>[2x]PNVAIIVAALKPALGIGYKGKMPWRLRKEIRYFKDVTTRTTKPNTRNAVIMGRKTWESIPQKFRPLP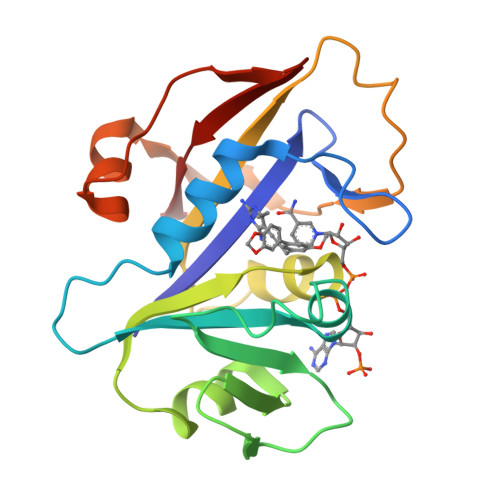DRLNIILSRSYENEIIDDNIIHASSIESSLNLVSDVERVFIIGGAEIYNELINNSLVSHLLITEIEHPSPESIEMDTFLKFPLESWTKQPKSELQKFVGDTVLEDDIKEGDFTYNYTLWTRK> TTQKKVVLSSFSIIGDITQNIAKDLVTVTTLVEAGNDAHSYQVTSADAIKIQNADLILCNGLHLEETYMKYFTNLKKGTKIITVTDGINPIGVSEDTSVDSEPNPHAWMSLTNAMIYIENIRKALTALDPSNAKKYELNAREYSEKIRNSILPLKTRIEKVDPEKRWFVTSEGCLVYLAEDFGFKSLYLWPINSDSERSPSMMRHAINQMRS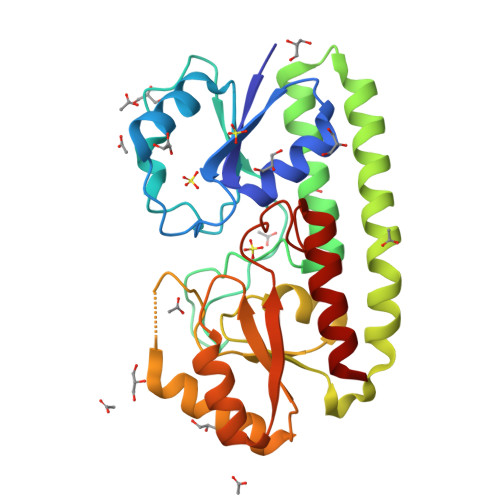HKIKFIFSESTNSDQPAKQVAYETNASYGGVLYVDSLSKPDGPAPTYLDLLRFSLTKIVDTLF(3S)-5-biphenyl-4-yl-3-hydroxypentanoic 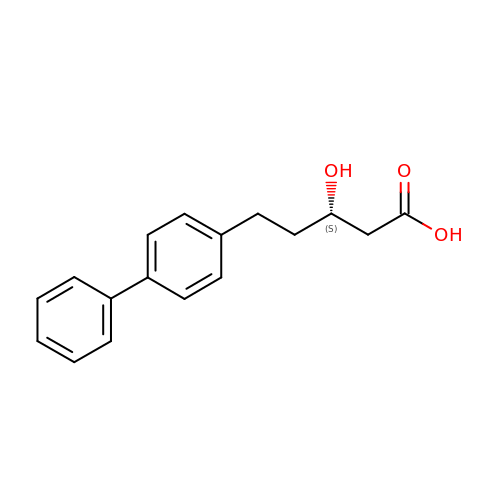acid | C17 H18 O3 | ILGSIIFHQGOKKV-INIZCTEOSA-N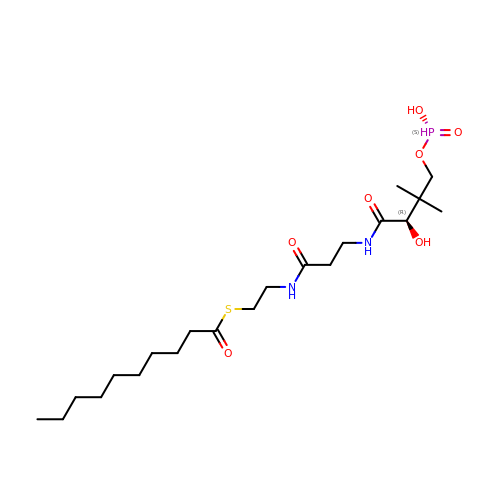S-(2-{[N-(2-HYDROXY-4-{[HYDROXY(OXIDO)PHOSPHINO]OXY}-3,3-DIMETHYLBUTANOYL)-BETA-ALANYL]AMINO}ETHYL) DECANETHIOATE | C21 H41 N2 O7 P S | BPRKYNVKIAROET-IBGZPJMESA-N> STSAASSSNYCNQMMKSRNLTKDRCKPVNTFVHESLADVQAVCSQKNVACKNGQTNCYQSY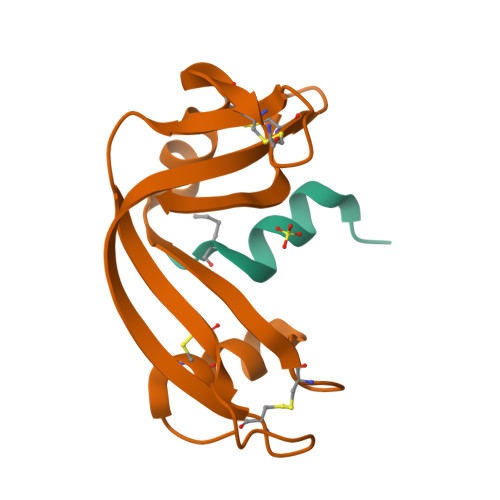STMSITDCRETGSSKYPNCAYKTTQANKHIIVACEGNPYVPVHFDASV;> KETAAAKFERQHLDSX>HMAKLRPYYEESQSAYDISDDFFALFLDPTWVYTCAYFERDDMTLEEAQLAKVDLALDKLNLEPGMTLLDVGCGWGGALVRAVEKYDVNVIGLTLSRNHYERSKDRLAAIGTQRRAEARLQGWEEFEENVDRIVSFEAFDAFKKERYLTFFERSYDILPDDGRMLLHSLFTYDRRWLHEQGIALTMSDLRFLKFLRESIFPGGELPSEPDIVDNAQAAGFTIEHVQLLQQHYARTLDAWAANLQAARERAIAV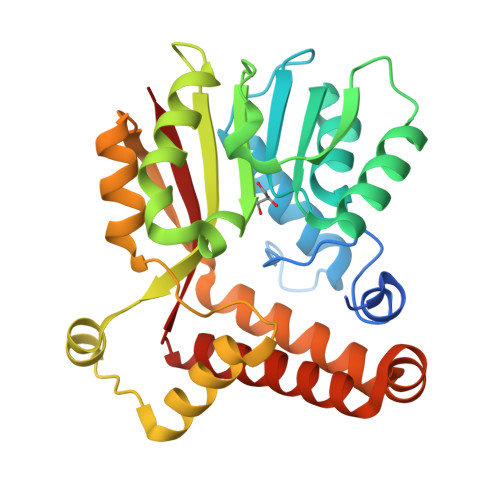QSEEVYNNFMHYLTGCAERFRRGLINVAQFTMTK[2x]>[2x]MAHHHHHHHRSSLTNVGNDRHAAGTDTDRARERDRRHLWHPWSSVRQPADDRPILVAGEGCRVRDVTGAGYLDAMASAMNSSCGYAHPALLEAARRQLELLPHFDLSAASHLPAGLAAERIAGLLPAGLERTFFVNSGSEATEAAVRIAHDHWTNRGEPRDRLVTFAAGYHGTTLVAQHLSGLPTNAIHGTA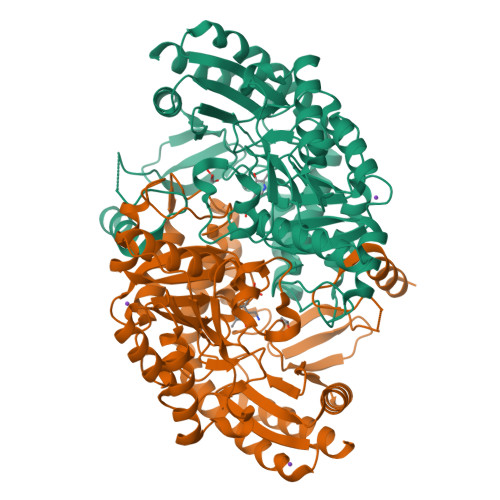PFPVTRVELPLEPAALRTPEALTLLADAFERAVLDGPPPAAVMVEPLLNVGGGVVLPDGFLRALRALCDRTGALLIVDEVFCGFGRTGRMFGFQHDGVTPDLVTMSKGISGGYVPFAALTTTDEVYRSFAADPLLGGLRYGHTTGGHAVACAVALAVLDVIEERGLVGSAARLGAELLAGLAPLAEHPEVTDVRGLGLVATVECRQPESAAALVAEAKRQGVLLRQQGRAVMAIPPLVIDAAEVAELVRAVEQAVARL> SPDKLKKVLDKLRLKRKDISEAAETVNKVVERLLRRMQKRESEFKGVEQLNTGSYYEHVKISAPNEFDVMFKLEVPRI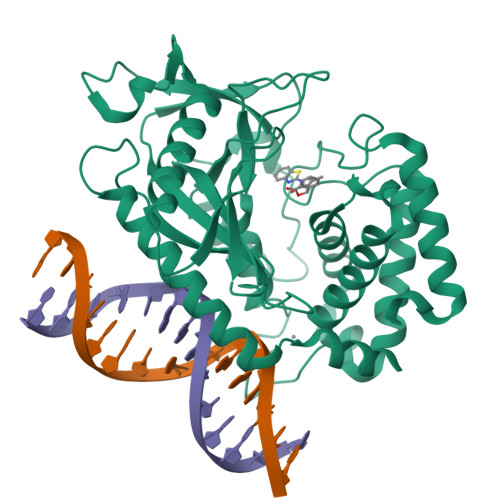ELQEYYETGAFYLVKFKRIPRGNPLSHFLEGEVLSATKMLSKFRKIIKEEVKEIKDIDVSVEKEKPGSPAVTLLIRNPEEISVDIILALESKGSWPISTKEGLPIQGWLGTKVRTNLRREPFYLVPKNAKDGNSFQGETWRLSFSHTEKYILNNHGIEKTCCESSGAKCCRKECLKLMKYLLEQLKKEFQELDAFCSYHVKTAIFHMWTQDPQDSQWDPRNLSSCFDKLLAFFLECLRTEKLDHYFIPKFNLFSQELIDRKSKEFLSKKIEYERNNGFPIFDKL>[2x]GSGPI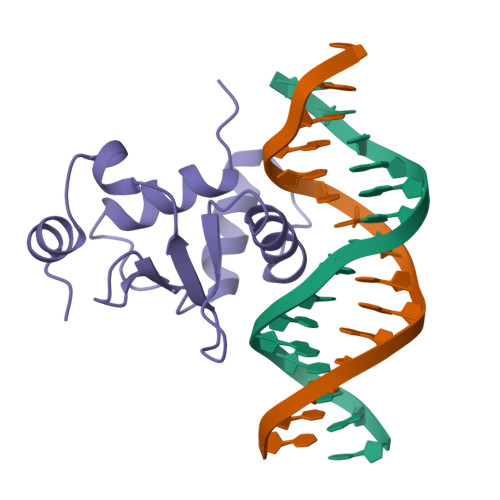QLWQFLLELLTDKSCQSFISWTGDGWEFKLSDPDEVARRWGKRKNKPKMNYEKLSRGLRYYYDKNIIHKTAGKRYVYRFVCDLQSLLGYTPEELHAMLDVKPDAD>[4x]MKLSDLISRWIDVEPSKNAQIILRDRYFMKDLDGNYLETKWEDVARRVARVVATAELLNPSYKKNEKLDRIKEWEDIFFRVLKARLFIPNSPTLFNAGLGVKHDLLWKPIDQMTLEDYEEIYRSRNHLHMLSACFVVPVGDSIEEIFEAVKEYALITKVGGGVGSNFSELRPKGSFVAGTHGKASGPVSFMHVFNSAISVVKQGSRRRGALMGILNINHPDIEEFIDAKKENTGEAVLNFFNLSVGFPMDKKEILKLYEEDGELELSHPRSTIRKKVKIRELFRKIATNAWKSGDPGLAFLGEMNKYYPLYPHRKINSTNPCGEIGLSDYEACNLGSIDV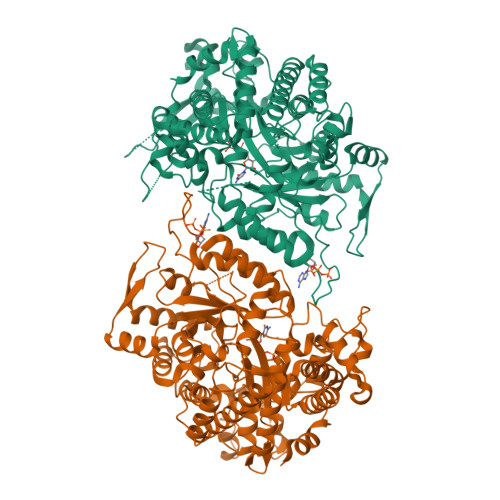AKFYNNGFVDLEALQELVQIAVRFLDNVIDVNVFPIDKITKAVKESRRLGLGIMGFADLLYKLEIPYNSQEARDFAANLMAFIALHAHRTSYELGKEKGNFPLLEISRYRTEDNFVPFAMGMSNYDDEIREVMKMTKEFRRNVALLTIAPTGSISNIADTSSGLEPNFLLAYTRFVTKEDGTKEPLLYVNQVLREKLNPEILKRIEKELIEKGSLKDIPDVPEKIKKVFVVALDIDPMDHLLMQDAFQRYVDNNISKTINMPQSATVDDVLNVYLEALRTNVRGITVYRDGSLQTQVLTKALKT~{tert}-butyl (2~{R})-2-[(4~{S})-6-(4-chlorophenyl)-8-methoxy-1-methyl-4~{H}-[1,2,4]triazolo[4,3-a][1,4]benzodiazepin-4-yl]pent-4-enoate 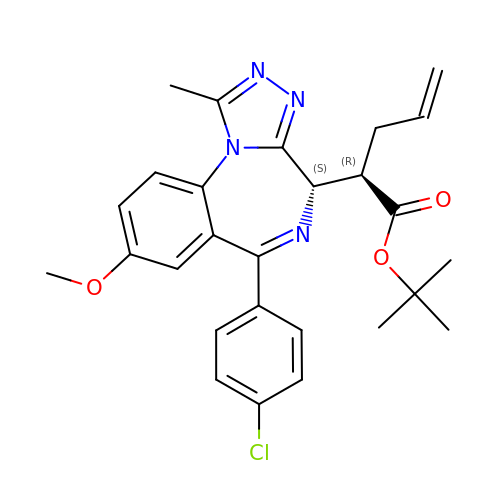| C27 H29 Cl N4 O3 | AUNFEHAUQMKWPP-YKSBVNFPSA-N> GHMIVIPPITDRKIRFALVGCGRIANNHFGALEKHADRAELIDVCDIDPAALKAAVERTGARGH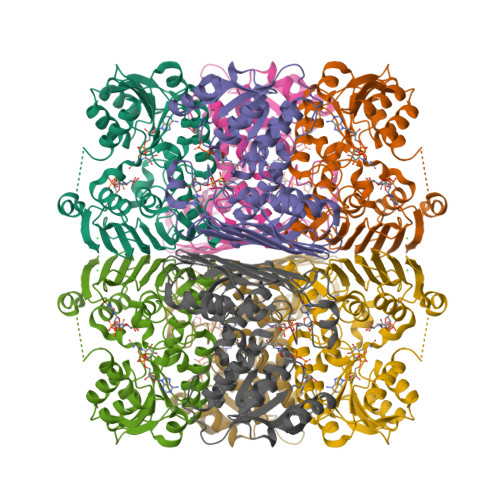ASLTDMLAQTDADIVILTTPSGLHPTQSIECSEAGFHVMTEKPMATRWEDGLEMVKAADKAKKHLFVVKQNRRNATLQLLKRAMQEKRFGRIYMVNVNVFWTRPQEYYDAAGWRGTWEFDGGAFMNQASHYVDLLDWLIGPVESVQAYTATLARNIEVEDTGTVSVKWRSGALGSMNVTMLTYPKNLEGSITILGEKGSVRVGGVAVNEIQHWEFSEPHAMDEEIKDASYATTSVYGFGHPLYYDNVIKTMRGEATPETDGREGLKSLELLIAMYLSARDGRRVSLPLDY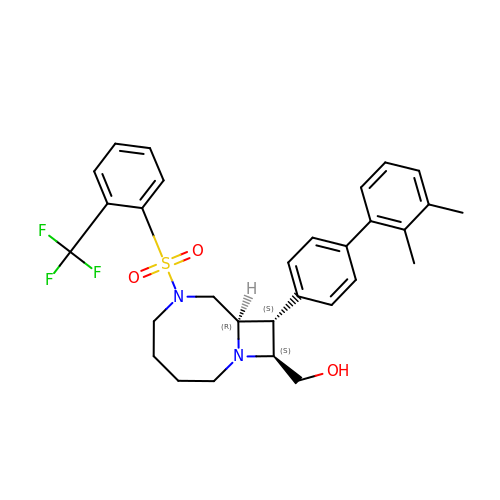[(8R,9S,10S)-9-(2',3'-dimethyl[1,1'-biphenyl]-4-yl)-6-{[2-(trifluoromethyl)phenyl]sulfonyl}-1,6-diazabicyclo[6.2.0]decan-10-yl]methanol | C30 H33 F3 N2 O3 S | OOPXWKPIZJCPGQ-GKRYNVPLSA-N>MYELTPEQRTLQTQARELAQSVFASTAVQTDLTEQYPWDNVAQLRDAGFMGMMLPTSVGGRGLSTLDTVIVIEEMAKACATMGRITVDSNLGAIGAITKYGSEEQIKLAADLVLAGDKPAICISEPNAGSAASEMTTRADKNGDHYILNGEKYWITGGGVSKLHLIFARVFDDGVEQGIGAFITVLDDHGPEGLKVGRRLYAMGVRGIPETHLEFHDLKIHKSMMITFPDGLKRGFAALMSAYNAQRVGAGAVALGIAQCAFEEGVAYLKRREQFGRPLAEFQGLQWMVADMSVQLEAARLMLRSAAVSGETFPDINKAAQAKIFAAETANKVTNDALQFFGSSGYGRHNPMERHVRDARMFTIA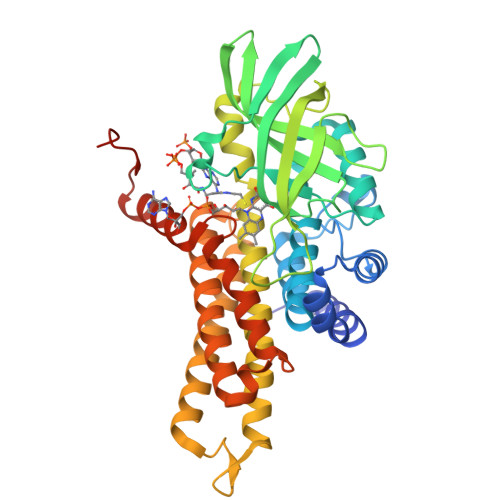GGTAQILRTQVASKILDMKLPQTRDGYLKAAQNSKR[6x]> MTENILRKSDEEIQKEITARVKALESMLIEQGILTTSMIDRMAEIYENEVGPHLGAKVVVKAWTDPEFKKRLLADGTEACKELGIGGLQGEDMMWVENTDEVHHVVVCTLCSCYPWPVLGLPPNWFKEPQYRSRVVREPRQLLKEEFGFEVPPSKEIKVWDSSSEMRFVVLPQRP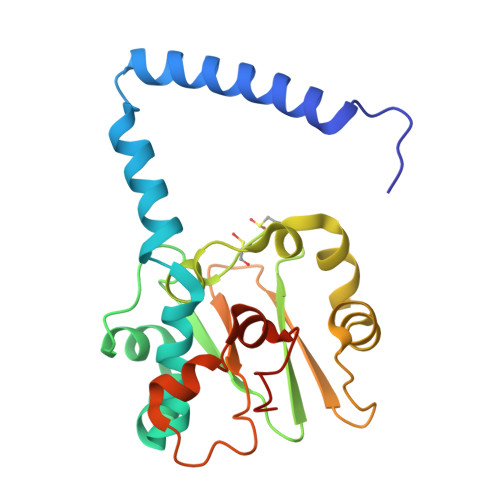AGTDGWSEEELATLVTRESMIGVEPAKAVAHHHHHH>MEKRMSTQQRAAGNACPTAAFSFDPARLAQRRRWAGAFAALCGLALSPSALLAEEHSQHQDHAVELAPSVVTGVAQSSPLTIVTNPKEPRQPVPASDGADYLKTIPGFAVIRNGGSNGDPVLRGMFGSRLNILTNGGMMLGACPNRMDAPTSYISPETYDKLTVIKGPQTVLWGPGASAGTILFEREPERFGELGSRVNASLLAGSNGRFDKVLDAAAGNRLGYLRFTGNHAQSDDYEDGAGNTVPSRWKKWNGDVAVGWTPDEDTLIELTAGKGDGEARYAGRGMDGSQFKRESLGLRFVKSNVSDVLEKVEAQVYYNYADAIMDNFRLRTPDPSSMMPMPMASQVDRRTLGGRLAATWRWDDFKLVTGVDAMRNEHRARGSKYDMMTDYYTDADQFPWSKDAVFHNYGAFGELTWFAAERDRLIGGLRLDRASVKDYRQTLKSGHMGHAMANPTANDTRADTLPSGFVRYEHDLADSPTTLYAGLGHAERFPDYWELFSPKRGPNGSVNAFDKIKPEKTTQLDFGLQYNGDKLQAWASGYVGVVQDFILFSYREGMMGSSTQATNVDARIMGGELGASYQLTGNWKTDASLAYAWGKNSSDDRALPQIPPLEARFGLTYEEGDWSAGSLWRVVAPQNRIARDQGNVVGKDFDKSAGFGVFSLNGAYRVTRNVKLSAGVDNLFDKDYTEHLNKAGDAGFGFSANETVPEPGRTFWTKVDFSF[4x]

Here, we show that Pseudomonas aeruginosa OprC is an outer membrane, TonB-dependent transporter that is conserved in many Proteobacteria and which mediates acquisition of both reduced and oxidised ionic copper via an unprecedented CxxxM-HxM metal binding site. As indicated by the successful structure solution, OprC contains a single bound copper and shows the typical fold of a TBDT, with a large 22-stranded β-barrel occluded by an N-terminal approximately 15 kDa plug domain that, like in other TBDTs, completely occludes the lumen of the barrel. The copper binding site comprises residues Cys143 and Met147 in the plug domain and His323 and Met325 in the barrel wall. The CxxxM-HxM configuration, which coordinates the copper in a tetrahedral manner, is highly unusual and has, to our knowledge, not been observed before in copper homeostasis proteins.

Since Cu(II) prefers histidine nitrogen as ligands and Cu(II) binding sites often contain one or more His residues, we also cocrystallised the H323A mutant with Cu(II) and Ag(I). One strong anomalous peak, at the high-affinity binding site, is observed with Cu(II), supporting the SEC data that the histidine is not required for Cu(II) binding. H323A (approximately 30%) and, in particular, M147A (approximately 60%), have relatively high occupancies after copper incubation and SEC, indicating that these residues contribute less towards binding. All 4 residues in the OprC binding site contribute to copper binding, but not to the same extent and, in some cases, not equally for both copper redox states. By contrast, removal of His323 still allows Cu(II) and Cu(I) binding.>[2x]ECGWRIGEAGTDPNLNHQQFRAKILSIWEECX;>[2x]SVRSSSRTPSDKPVAHVVANPQAEGQLQWLNRRANALLANGVELRDNQLVVPSEGLYLIYSQVLFKGQGCPSTHVLLT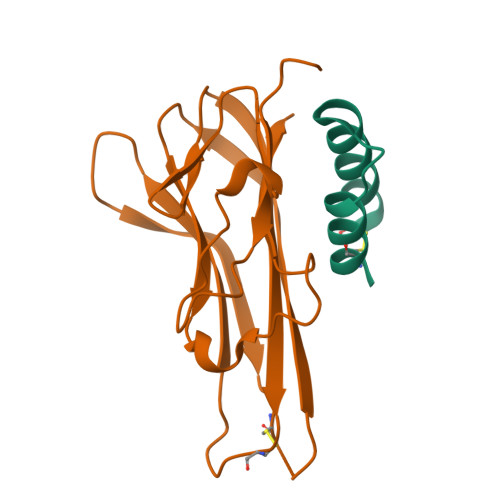HTISRIAVSYQTKVNLLSAIKSPCQRETPEGAEAKPWYEPIYLGGVFQLEKGDRLSAEINRPDYLDFAESGQVYFGIIAL>GHMSIKPKIMISSLDAERLEILLETLSQNAFPGRDDLE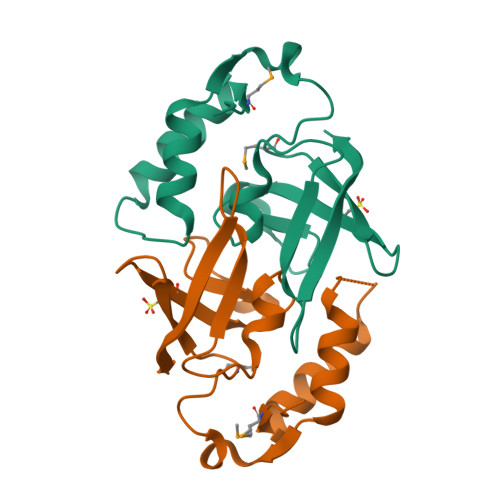AELARAEVVDPEEIPPTVVTMNSTVRFRVESSAEEFCLTLVYPKDVDTSGEKISILAPVGSALLGLAQGDEIEWPKPGGGVLRVRIVEVTYQPERSGEYYRGS[4x]> GAHMDCHLSDMLQQLHSVNASKPSERGLVRQEEAEDPACIPIFWVSKWVDYSDKYGLGYQLCDNSVGVLFNDSTRLILYNDGDSLQYIERDGTESYLTVSSHPNSLMKKITLLKYFRNYMSEHLLKAGANITPREGDELARLPYLRTWFRTRSAIILHLSNGSVQINFFQDHTKLILCPLMAAVTYIDEK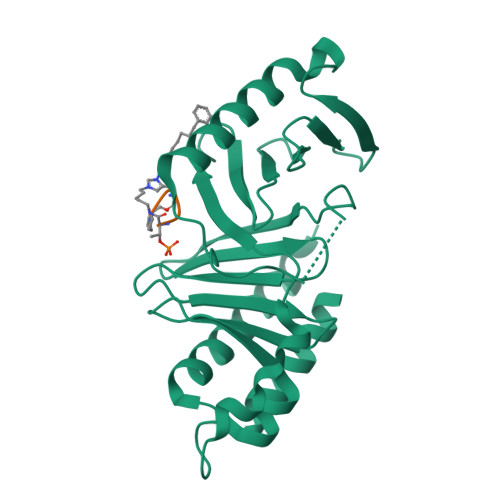RDFRTYRLSLLEEYGCCKELASRLRYARTMVDKLLSSRSASNRLKAS;> PLHST> GECGDMFNGDDSSVVRRSANYPANLWDYDFLQSLGRHSSVTEEHVGLAEKLKGEVKSLITGPMEPLAKLEFIDSVRRLGLKYQFETEMKEALANISKDGYDSWWVDNLRATALRFRLLRENGIFVPQDVFERFQNKETGKFKNELCEDVKGLLNLYEASFLGWEGEDILDEARTFSTAQLKNVEKKISSPNLAKIVHHALDLPLHWRAIRYEARWFIDIYEDEEDMNPTLLKYAKLDFNIVQSFHQAEIGRLARWWVGTGLDKLPFARNGLIQSYMYAIGMLFEPHLGEVREMEAKVGALITTIDD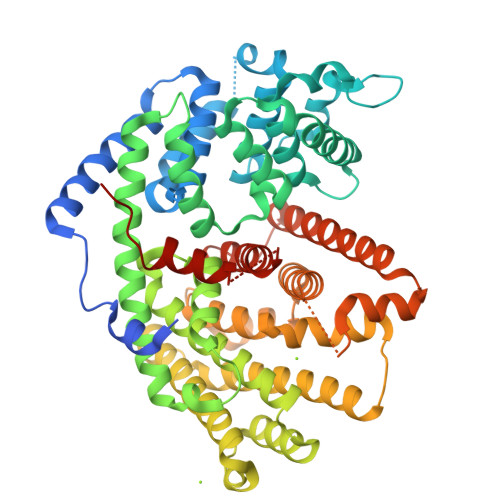VYDVYGTMEELELFTDITERWDINRVDQLPRNIRMPLLTMFNTSNDIGYWALKERGFNGIPYTAKVWADQLKSYTKEAKWFHEGHKPTLEEYLENALVSIGFPNLLVTSYLLTVDNPTKEKLDYVDSLPLFVRASCILCRIINDLGTSPDEMERGDNLKSIQCYMNETGASQEVAREHIEGLVRMWWKRLNKCLFEPSPFTEPFLSFTINVVRGSHFFYQYGDGYGNAESWTKNQGMSVLIHPITLDEE>VSQPAPMSPKVTVGGSVGGVSLQARQAQLRLRLYAVVQGRMQTIAERRYRVSGLPLRYAFDLEVDRLEGEAL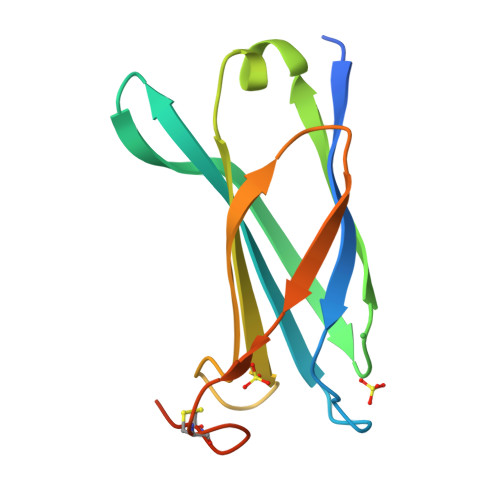YLRTELSWVGVAAVQASAWQQVAAGVDERVRLVRRDCFPNCTAARPEERSGND[3x]>MNMTELKGALIGCGFFAVNQMHAWKDVKGAGIAAICDRDPKRLKLVGDQFGIERRYGDAAALFADGGFDFVDIATTVQSHRALVEMAAAHKVPAICQKPFAKSLSDAKAMVRTCENADIPLMVHENFRWQTPIQAVKAVLESGAIGEPFWGRFSFRSGFDVFSGQPYLAEGERFIIEDLGIHTLDIARFILGDVATLTARTKRVNPKIKGEDVATILLDHQNGATSIVDVSYATKLGTEPFPETLIDIDGTQGTIRLSQGYRLE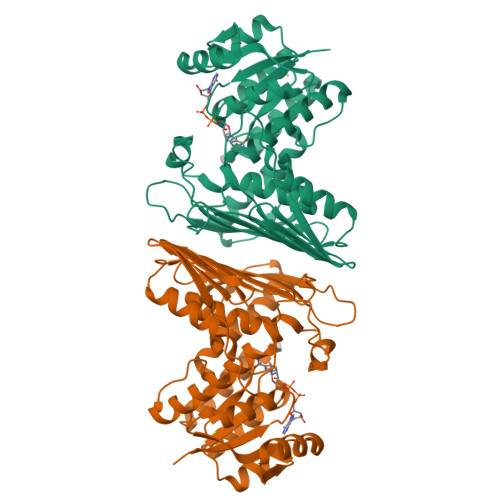VTGPNGMTISDASPQLLSWASRPWHNIQESVLAIQQHWTDRLSSGGETSTSGADNLKTFALVEAAYESAANGRTVDIGAML[2x]>AASIFAAVPRAPPVAVFKLTADFREDGDSRKVNLGVGAYRTDEGQPWVLPVVRKVEQLIAGNGSLNHEYLPILGLPEFRANASRIALGDDSPAIAQKRVGSVQGLGGTGALRIGAEFLRRWYNGNNNTATPVYVSSPTWENHNSVFMDAGFKDIRTYRYWDAAKRGLDLQGLLSDMEKAPEFSIFILHACAHNPTGTDPTPDEWKQIAAVMKRRCLFPFFDSAYQGFASGNLEKDAWAVRYFVSEGFELFCAQSFSKNFGLYNERVGNLSVVGKDEDNVQRVLSQMEKIVRTTWSNPPSQGARIVATTLTSPQLFAEWKDNVKTMADRVLLMRSELRSRLESLGTPGTWNHITDQ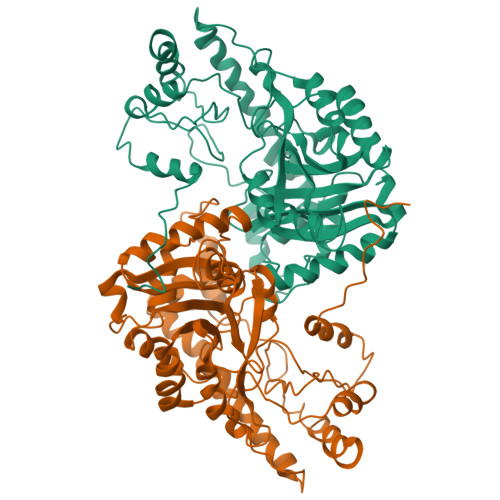IGMFSFTGLNPKQVEYMIKEKHIYLMASGRINMCGLTTKNLDYVAKSIHEAVTKIQ[2x]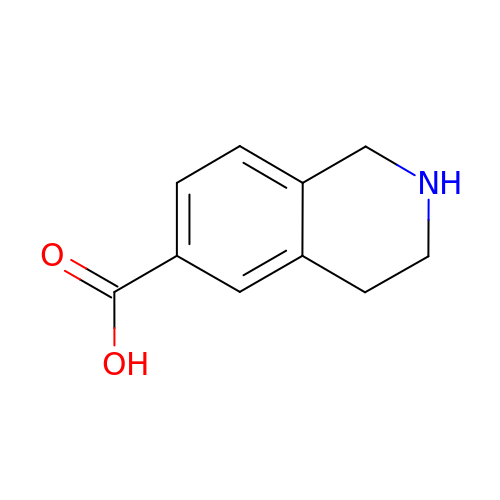1,2,3,4-tetrahydroisoquinoline-6-carboxylic acid | C10 H11 N O2 | QEMYLDYQDFRTRT-UHFFFAOYSA-N>MGSIDSTNVAMSNSPVGEFKPLEAEEFRKQAHRMVDFIADYYKNVETYPVLSEVEPGYLRKRIPETAPYLPEPLDDIMKDIQKDIIPGMTNWMSPNFYAFFPATVSSAAFLGEMLSTALNSVGFTWVSSPAATELEMIVMDWLAQILKLPKSFMFSGTGGGVIQNTTSESILCTIIAARERALEKLGPDSIGKLVCYGSDQTHTMFPKTCKLAGIYPNNIRLIPTTVETDFGISPQVLRKMVEDDVAAGYVPLFLCATLGTTSTTATDPVDSLSEIANEFGIWIHVDAAYAGSACICPEFRHYLDGIERVDSLSLSPHKWLLAYLDCTCLWVKQPHLLLRALTTNPEYLKNKQ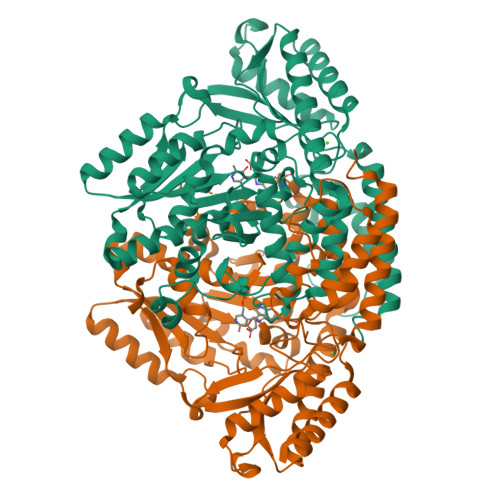SDLDKVVDFKNWQIATGRKFRSLKLWLILRSYGVVNLQSHIRSDVAMAKMFEEWVRSDSRFEIVVPRNFSLVCFRLKPDVSSLHVEEVNKKLLDMLNSTGRVYMTHTIVGGIYMLRLAVGSSLTEEHHVRRVWDLIQKLTDDLLKEA[4x]> AHHHHHHGSKVV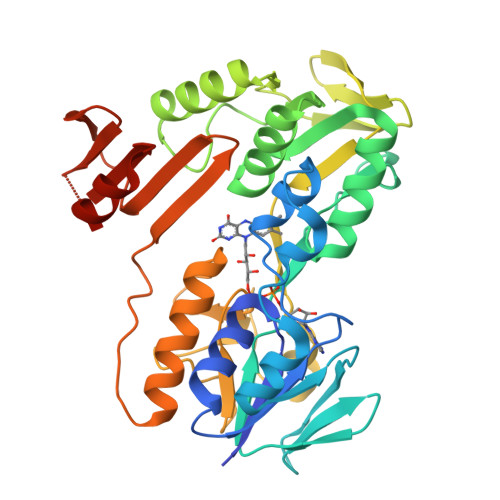IVGNGPGGFELAKQLSQTYEVTVIDKEPVPYYSKPMLSHYIAGFIPRNRLFPYSLDWYRKRGIEIRLAEEAKLIDRGRKVVITEKGEVPYDTLVLATGARAREPQIKGKEYLLTLRTIFDADRIKESIENSGEAIIIGGGFIGLELAGNLAEAGYHVKLIHRGAMFLGLDEELSNMIKDMLEETGVKFFLNSELLEANEEGVLTNSGFIEGKVKICAIGIVPNVDLARRSGIHTGRGILIDDNFRTSAKDVYAIGDCAEYSGIIAGTAKAAMEQARVLADILKGEPRRYNFKFRSTVFKFGKLQIAIIGNTKGEGKWIEDNTKVFYENGKIIGAVVFNDIRKATKLEKEILDFYS>[2x]MNTFDKHDLSGFVGKHLVYTYDNGWEYEIYVKNEN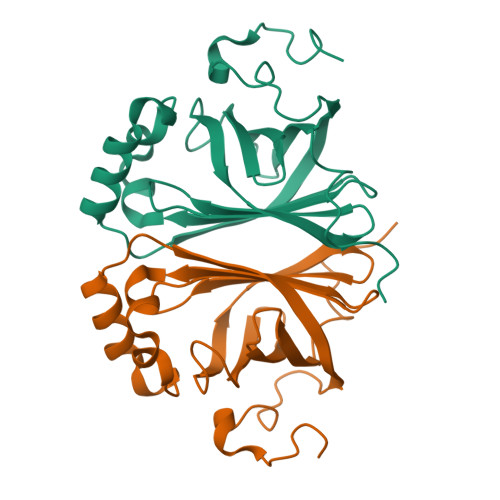TLDYRIHSGLVGNRWVKDQQAYIVRVGESIYKISWTEPTGTDVSLIVNLGDSLFHGTIFFPRWVMNNPEKTVCFQNDHIPLMNSYRDAGPAYPTEVIDEFATITFVRDCGANNESVIACAASELPKNFPDNLK>QQASTLPDLAEQFAPPDVAPPLLIKLVEAIEKKGLECSTLYRTQSSSNPAELRQLLDCDTASLDLEMFDVHVLADAFKRYLLDLPNPVIPVAVSSELISLAPEVQSSKEYIQLLKKLIRSPSIPHQYWLTLQYLLKHFFKLSQTSSKNLLNARVLSELFSPLLFRFPAASSENTEHLIKIIEILISTEWNERQ[2x]

The N-terminal domains of p85α include an SH3 domain, capable of binding to proline-rich sequences, and a BH (breakpoint cluster region homology) domain. The BH domain can bind to and regulate several GTPases including Rab5, Rac1 and Cdc42. In addition, the p85α BH domain, either alone or together with the SH3 domain, can bind to and positively regulate PTEN activity. The p85α BH domain also exhibits Rab5 GAP activity to stimulate Rab5-mediated GTP hydrolysis required to inactivate Rab5-mediated protein trafficking functions.

To determine if the patient-derived p85α BH domain mutations impacted the overall folded structure of the BH domain, several of these BH domain mutants were crystalized and their structures were determined using X-ray crystallography. X-ray diffraction data collection and structure refinement statistics for bovine p85α (105–319) mutants (E137K, E217K, R262T, E297K) are provided in Supplementary Table S1. Three BH domain mutants, I177N, E217K and E297K, all showed significantly increased Rab5-GAP activity, whereas the E137K mutant had reduced activity. The location of cancer patient-derived p85α BH mutations with significant impacts on Rab5 binding (I177, E217) and/or regulation (E137, I177, E217, E297) are shown in the modeled p85α BH domain: Rab5 complex. These mutation sites are located in regions of the p85α BH domain, well away from the Rab5 binding pocket. Further, crystal structure determinations for several of these mutant BH domains indicated that no major structural alterations were present. No significant differences in protein flexibility were observed for any of the mutant proteins, suggesting that the mutations did not alter the rigidity of the domain.(2S)-{[(3-{[(2-chloro-6-methylphenyl)carbamoyl]amino}naphthalen-2-yl)carbonyl]amino}(phenyl)ethanoic acid | C27 H22 Cl N3 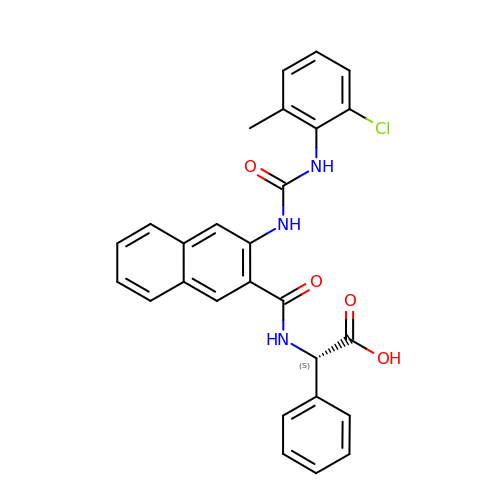O4 | KRIVDSIBMDCVLL-DEOSSOPVSA-N> MACWPQLRLLLWKNLTFRRRQTCQLLLEVAWPLFIFLILISVRLSYPPYEQHECHFPNKAMPSAGTLPWVQGIICNANNPCFRYPTPGEAPGVVGNFNKSIVARLFSDARRLLLYSQKDTSMKDMRKVLRTLQQIKKSSSNLKLQDFLVDNETFSGFLYHNLSLPKSTVDKMLRADVILHKVFLQGYQLHLTSLCNGSKSEEMIQLGDQEVSELCGLPREKLAAAERVLRSNMDILKPILRTLNSTSPFPSKELAEATKTLLHSLGTLAQELFSMRSWSDMRQEVMFLTNVNSSSSSTQIYQAVSRIVCGHPEGGGLKIKSLNWYEDNNYKALFGGNGTEEDAETFYDNSTTPYCNDLMKNLESSPLSRIIWKALKPLLVGKILYTPDTPATRQVMAEVNKTFQELAVFHDLEGMWEELSPKIWTFMENSQEMDLVRMLLDSRDNDHFWEQQLDGLDWTAQDIVAFLAKHPEDVQSSNGSVYTWREAFNETNQAIRTISRFMECVNLNKLEPIATEVWLINKSMELLDERKFWAGIVFTGITPGSIELPHHVKYKIRMDIDNVERTNKIKDGYWDPGPRADPFEDMRYVWGGFAYLQDVVEQAIIRVLTGTEKKTGVYMQQMPYPCYVDDIFLRVMSRSMPLFMTLAWIYSVAVIIKGIVYEKEARLKETMRIMGLDNSILWFSWFISSLIPLLVSAGLLVVILKLGNLLPYSDPSVVFVFLSVFAVVTILQCFLISTLFSRANLAAACGGIIYFTLYLPYVLCVAWRDYVGFTLKIFASLLSPVAFGFGCEYFALFEEQGIGVQWDNLFESPVEEDGFNLTTSVSMMLFDTFLYGVMTWYIEAVFPGQYGIPRPWYFPCTKSYWFGEESDEKSHPGSNQKRISEICMEEEPTHLKLGVSIQNLVKVYRDGMKVAVDGLALNFYEGQITSFLGHNGAGKTTTMSILTGLFPPTSGTAYILGKDIRSEMSTIRQNLGVCPQHNVLFDMLTVEEHIWFYARLKGLSEKHVKAEMEQMALDVGLPSSKLKSKTSQLSGGMQRKLSVALAFVGGSKVVILDEPTAGVDPYSRRGIWELLLKYRQGRTIILSTHHMDEADVLGDRIAIISHGKLCCVGSSLFLKNQLGTGYYLTLVKKDVESSLSSCRNSSSTVSYLKKEDSVSQSSSDAGLGSDHESDTLTIDVSAISNLIRKHVSEARLVEDIGHELTYVLPYEAAKEGAFVELFHEIDDRLSDLGI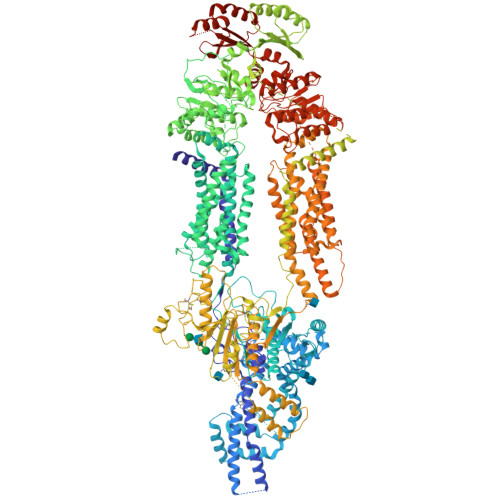SSYGISETTLEEIFLKVAEESGVDAETSDGTLPARRNRRAFGDKQSCLRPFTEDDAADPNDSDIDPESRETDLLSGMDGKGSYQVKGWKLTQQQFVALLWKRLLIARRSRKGFFAQIVLPAVFVCIALVFSLIVPPFGKYPSLELQPWMYNEQYTFVSNDAPEDTGTLELLNALTKDPGFGTRCMEGNPIPDTPCQAGEEEWTTAPVPQTIMDLFQNGNWTMQNPSPACQCSSDKIKKMLPVCPPGAGGLPPPQRKQNTADILQDLTGRNISDYLVKTYVQIIAKSLKNKIWVNEFRYGGFSLGVSNTQALPPSQEVNDAIKQMKKHLKLAKDSSADRFLNSLGRFMTGLDTKNNVKVWFNNKGWHAISSFLNVINNAILRANLQKGENPSHYGITAFNHPLNLTKQQLSEVALMTTSVDVLVSICVIFAMSFVPASFVVFLIQERVSKAKHLQFISGVKPVIYWLSNFVWDMCNYVVPATLVIIIFICFQQKSYVSSTNLPVLALLLLLYGWSITPLMYPASFVFKIPSTAYVVLTSVNLFIGINGSVATFVLELFTDNKLNNINDILKSVFLIFPHFCLGRGLIDMVKNQAMADALERFGENRFVSPLSWDLVGRNLFAMAVEGVVFFLITVLIQYRFFIRPRPVNAKLSPLNDEDEDVRRERQRILDGGGQNDILEIKELTKIYRRKRKPAVDRICVGIPPGECFGLLGVNGAGKSSTFKMLTGDTTVTRGDAFLNKNSILSNIHEVHQNMGYCPQFDAITELLTGREHVEFFALLRGVPEKEVGKVGEWAIRKLGLVKYGEKYAGNYSGGNKRKLSTAMALIGGPPVVFLDEPTTGMDPKARRFLWNCALSVVKEGRSVVLTSHSMEECEALCTRMAIMVNGRFRCLGSVQHLKNRFGDGYTIVVRIAGSNPDLKPVQDFFGLAFPGSVLKEKHRNMLQYQLPSSLSSLARIFSILSQSKKRLHIEDYSVSQTTLDQVFVNFAKDQSDDDHLKDLSLHKNQTVVDVAVLTSFLQDEKVKESYVGDYKDDDDK> GPKLAALDPIASQFSQLRTISKADAESEELGFKDAADHHT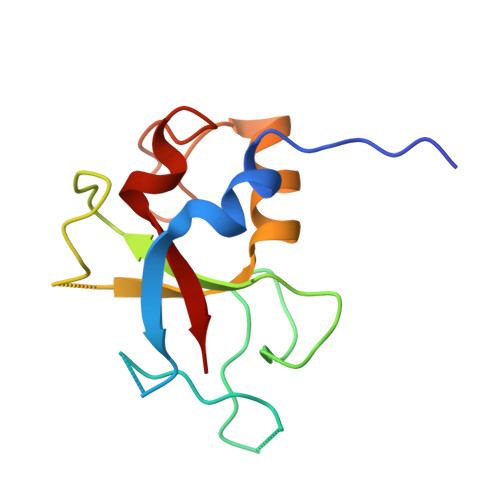DDVTHCLFGGELSLSNPDQQVIGLAGNPTDTSQPYSQEGNKDLAFMDMKKLAQFLAGKPEHPMTRETLNAENIAKYAFRIVP> GSTKETAFVEVVLFESSPSGDYTTYTTGLTGRF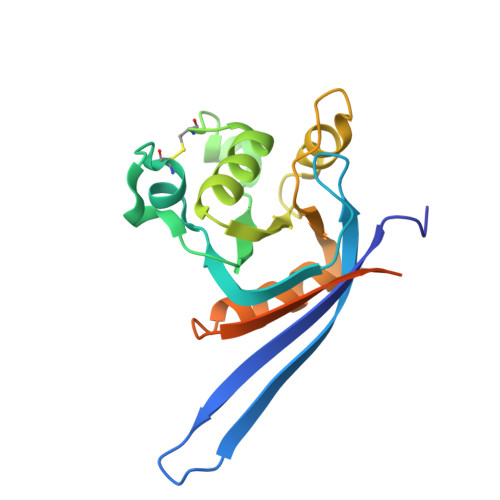SRAGATLSAEGEIVQMHPLGLCNNNDEEDLYEYGWVGVVKLEQPELDPKPCLTVLGKAKRAVQRGATAVIFDVSENPEAIDQLNQGSEDPLKRPVVYVKGADAIKLMNIVNKQKVARARIQHRPPRQPTEYFDMGNSDYKDDDDK> EPKMPPAVADAKASGIARFNAYTQYFPEATLITQPHATGHVGNFFFTHWKDGGSAALDLDAKGNFSVSWQGGGYNYVGGPGWHFGDKNRVIGYRFNQDSGASYITLYGWGYDKSMPATDPAHLVEYYILQRWTYDPSQ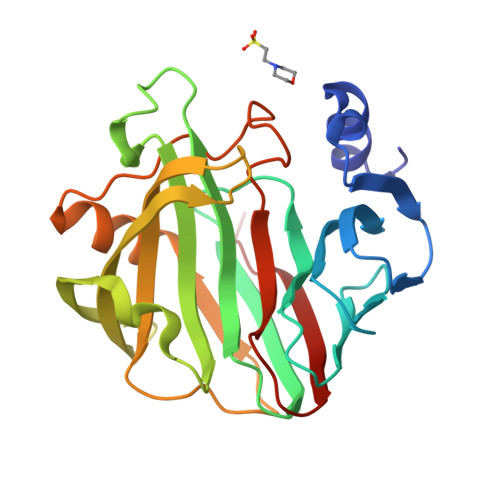DGIYGKTFVSNGIEYSTYRSIRKVKPSINGPTTFYQYWSKPSAQQELGKDHKIIFADHVKAWADTGWILPDMNNFDASDDPTYQVLAVEVFNPQKNGTASGQVWDETPR>[3x]MSTTLAIVRLDPGLPLPSRAHDGDAGVD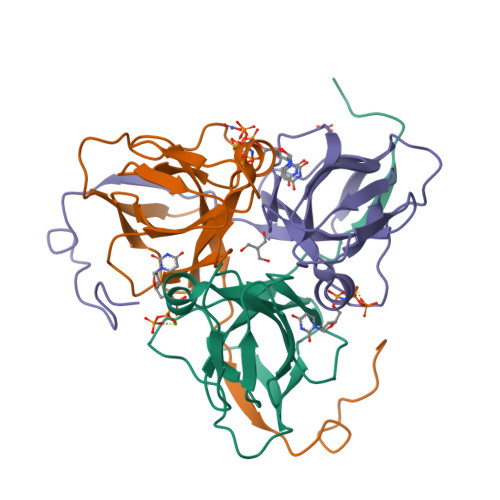LYSAEDVELAPGRRALVRTGVAVAVPFGMVGLVHPRSGLATRVGLSIVNSPGTIDAGYRGEIKVALINLDPAAPIVVHRGDRIAQLLVQRVELVELVEVSSFDEAGLASTSRGDGGHGSSGGHASLGVPRGAAALEHHHHHH> MSAAQSAVRSHAEAVQVSRTIDWMALFVVFFVIVGSYHIHAMLTMGDWDFWSDWKDRRLWVTVTPIVLVTFPAAVQSYLWERYRLPWGATVCVLGLLLGEWINRYFNFWGWTYFPINFVFPASLVPGA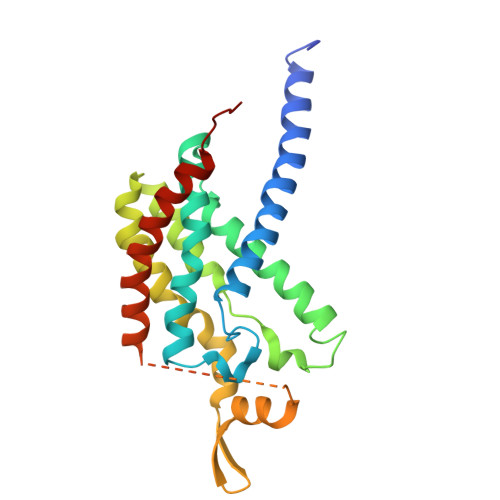IILDTVLMLSGSYLFTAIVGAMGWGLIFYPGNWPIIAPLHVPVEYNGMLMSIADIQGYNYVRTGTPEYIRMVEKGTLRTFGKDVAPVSAFFSAFMSILIYFMWHFIGRWFSNERFLQST> ISGGDAI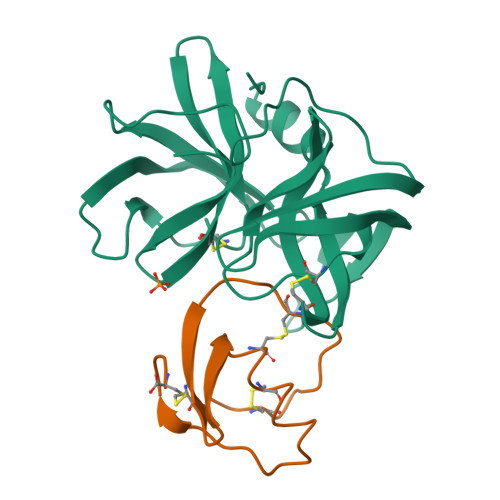YSSTGRCSLGFNVRSGSTYYFLTAGHCTDGATTWWANSARTTVLGTTSGSSFPNNDYGIVRYTNTTIPKDGTVGGQDITSAANATVGMAVTRRGSTTGTHSGSVTALNATVNYGGGDVVYGMIRTNVCAEPGDSGGPLYSGTRAIGLTSGGSGNCSSGGTTFFQPVTEALSAYGVSVY;> VDCSEYPKPACTQEYRPLCGSDNKTYGNKCNFCNAVVESNGTLTLSHFGKC> APAVADKADNAFMMICTALVLFMTIPGIALFYGGLIRGKNVLSMLTQVTVTFALVCILWVVYGYSLAFGEGNNFFGNINWLMLKNIELTAVMGSIYQYIHVAFQGSFACITVGLIVGALAERIRFSAVLIFVVVWLTLSYIPIAHMVWGGGLLASHGALDFAGGTVVHINAAIAGLVGAYLIGKRVGFGKEAFKPHNLPMVFTGTAILYIGWFGFNAGSAGTANEIAALAFVNTVVATAAAILGWIFGEWALRGKPSLLGACSGAIAGLVGVTPACGYIGVGGALIIGVVAGLAGLWGVTMLKRLLRVDDPCDVFGVHGVCGIVGCIMTGIFAASSLGGVGFAEGVTMGHQLLVQLE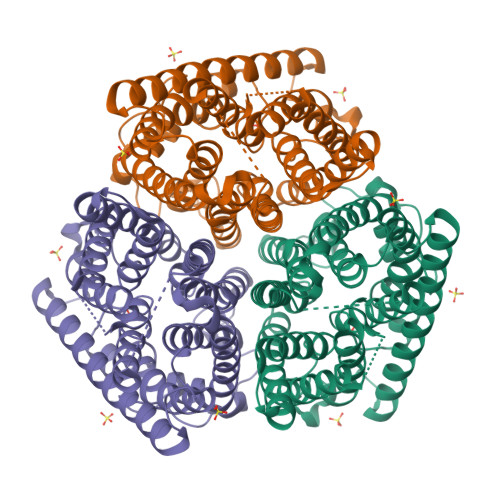SIAITIVWSGVVAFIGYKLADLTVGLRVPEEQEREGLDVNSHGENAYNADQAQQPAQADLE> PISPIETVPVKLKPGMDGPKVKQWPLTEEKIKALVEICTELEKEGKISKIGPENPYNTPVFAIKKKDSTKWRKLVDFRELNKRTQDFWEVQLGIPHPAGLKKKKSVTVLDVGDAYFSVPLDEDFRKYTAFTIPSINNETPGIRYQYNVLPQGWKGSPAIFQSSMTKILEPFRKQNPDIVIYQYMDDLYVGSDLEIGQHRTKIEELRQHLLRWGLYTPDKKHQKEPPFLWMGYELHPDKWTVQPIVLPEKDSWTVNDIQKLVGKLNWASQIYPGIKVRQLCKLLRGTKALTEVIPLTEEAELELAENREILKEPVHGVYYDPSKDLIAEIQKQGQGQWTYQIYQEPFKNLKTGKYARMRGAHTNDVKQLT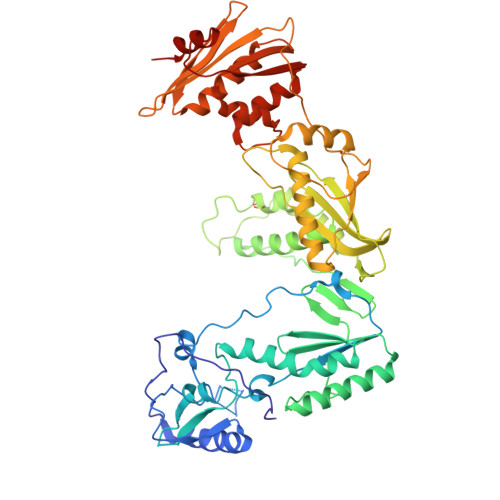EAVQKITTESIVIWGKTPKFKLPIQKETWETWWTEYWQATWIPEWEFVNTPPLVKLWYQLEKEPIVGAETFYVDGAANRETKLGKAGYVTNRGRQKVVTLTDTTNQKTELQAIYLALQDSGLEVNIVTDSQYALGIIQAQPDQSESELVNQIIEQLIKKEKVYLAWVPAHKGIGGNEQVDKLVSAGIRKVL>MELIKGQALFLELDKKDFLSLKNNDKNIPTFA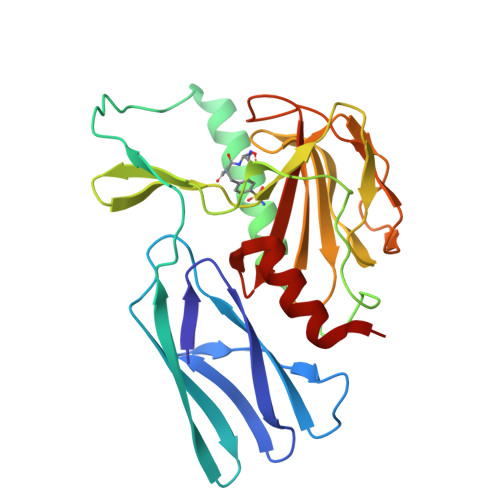HPKNQEKILAIFSLPYKNPPQNTKLIAFYKDKKEEIFIKTLEGNYKSEKLQVENKKIFPPKTIQERIAKELKEANAIYSSYTPKALFNGAFNIPLNSFITSDFGKARTFNEKVASYHSGTDFRAATGTPIYAANSGVVKIAKDRYFAGNSVVIDHGFGIYSQYYHLSKIDVKVGQKIKKGELIGLSGASGRVSGPALHFGILAGGKQVDPLDFVSKFNAIFQL[2x]>[2x]MMKPEDVIKEQCARAKVVAELWHGFTGGAPKAALENLVVEFN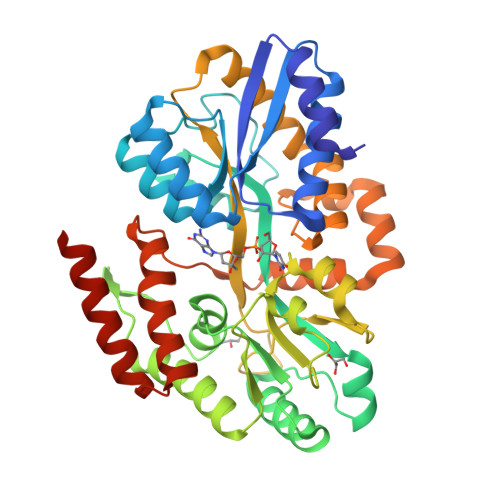KAQQGRCVRPVPQGGYRDLSTKIKAAFAAGKVPTMAQAFENNIALYLEAKALLPIESLGVKLQGVNLTFLNAVRFGGVVYGVPFNKSIQVLYYNKDLLKKHGVPVPATLEEFVAAAKKLSRAEGGPVYWFQPDASTFAYFFFNLGGSYLKDGKLVLNSKEAVEALTLLQNGVKEGWAKPITSGYINQNLGSGPYAFSVDTSAGYTYYLRAAKFDLGVATLPGRTKGQPGYGLVAGTNLVVFRQASKEEQAVAKDFLEFVLSPRAQAVFATATGYVPVTEGALKDPVYQAYAAENPDYATIVRQSRYAKFEPALAEWEQIRFDILGQAIKEAILNKADPKAALDRAQKLAEDLLSSRTRHHHHHH> VTLDGGAVAAPDQYGAKVAAEILKKGGNAVDAAVATAFTLAVTYPEAGNIGGGGFMTLYVDGKPYFLDYREIAPKAATKTMYLNEKGEVIENLSLVGAKAAGVPGTVMGLWEAHQRFGKLKWSELLTPAIGYAQTGFKVADQQYQYRQDAIALFNGKTNFGDYFGTMKPGEVFKQPELAKTLERIADKGPDDFYKGETAKLLIAQMKQDGGLI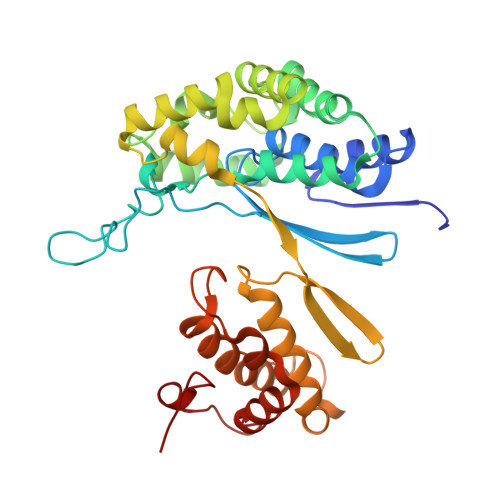TSDDLVDYQAKWREPMRIDWQGNTLYTAPLPSSGGIALAQLIGIKEQRAADFKGVELNSAKYIHLLSEIEKRVFADRADYLGDPQFSKVPVAQLTDPKYIAKRAGEVNPDAISATEKVRPGLEPHQ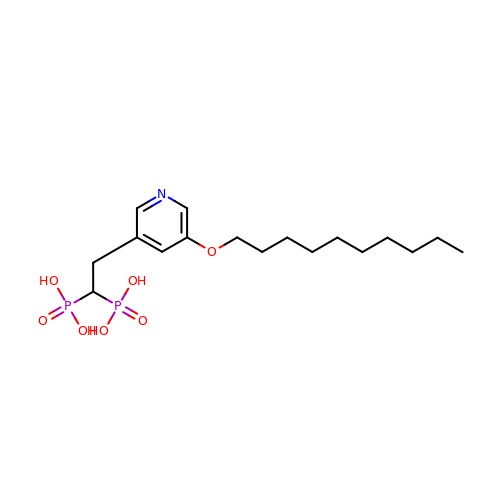{2-[5-(decyloxy)pyridin-3-yl]ethane-1,1-diyl}bis(phosphonic acid) | C17 H31 N O7 P2 | CXNUSEYMNGPVLV-UHFFFAOYSA-N>QAKHKQRKRLKSSCKRHPLYVDFSDVGWNDWIV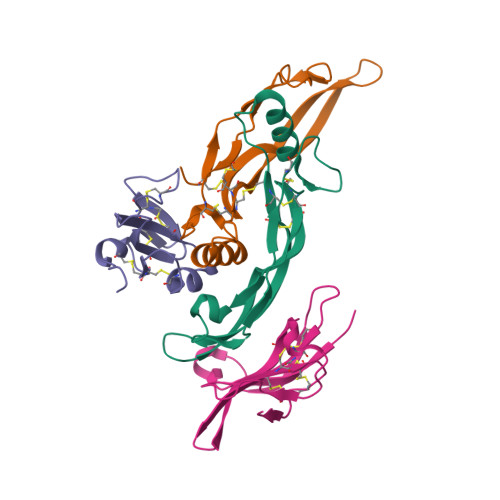APPGYHAFYCHGECPFPLADHLNSTNHAIVQTLVNSVNSKIPKACCVPTELSAISMLYLDENEKVVLKNYQDMVVEGCGCR[2x];> QNLDSMLHGTGMKSDSDQKKSENGVTLAPEDTLPFLKCYCSGHCPDDAINNTCITNGHCFAIIEEDDQGETTLASGCMKYEGSDFQCKDSPKAQLRRTIECCRTNLCNQYLQPTLPPVVIGPFFDGSIR;> SGRGEAETRECIYYNANWELERTNQSGLERCEGEQDKRLHCYASWRNSSGTIELVKKGCWLDDFNCYDRQECVATEENPQVYFCCCEGNFCNERFTHL> MHHHHHHHHMTNNGNEPNLTLSDLYDKDVVYTSRPSYISNPWLKPDEHQSNFLTGRELLIANQLPVIVHEASATDKLHQLFQVIGKEVPNSIYTFNNQQSYENLIKQLAHKENKKIYFQYIHDETILNQQYYALDKTLFVALNNKARIPEWTNGKFLPKRKVVKIEQFENEIKNWEFPLVIKPGDDLPTAGGYGVMICYHDADLQKAITRIKEATAETNSLIIEQKIEEKANYCVQFAYSESLGIQYLGAATQLTDKYGFYNGNENTTNVPEHVIEAGRQIMENGVNQGFFGVAGFDLLVDEDDNVYAIDLNFRQNGSTSMLLLANELNSGYQKFYSYHSKGDNTHFFNTILKYVKEGSLYPL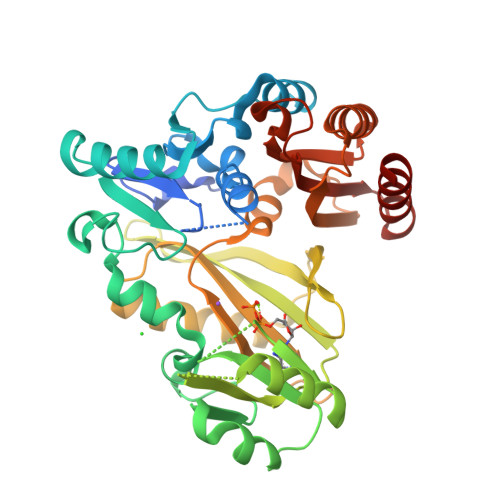SYYDGDWYGEDKVKSRFGCIWHGDSKETVLENERAFLAELEHY(1R,2S,3R,5Z,7E)-17-{(1R)-1-[(2-ethyl-2-hydroxybutyl)sulfanyl]ethyl}-2-(2-hydroxyethoxy)-9,10-secoestra-5,7,16-triene-1,3-diol 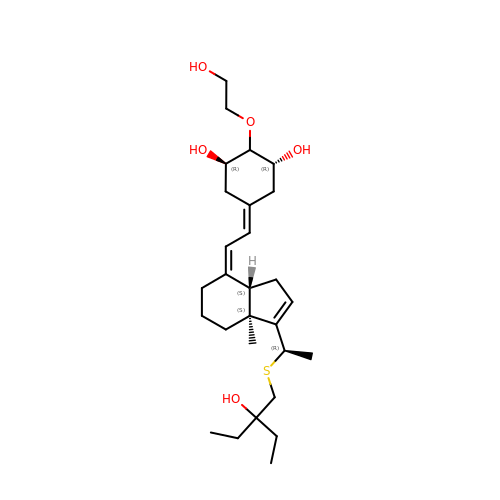| C28 H46 O5 S | DUIYWCMQVXJTIP-XXAWZNHHSA-N>[2x]AGTYNYGEALQKSIMFYEFQRSGDLPADKRDNWRDDSGMKDGSDVGVDLTGGWYDAGDHVKFNLPMSYTSAMLAWSLYEDKDAYDKSGQTKYIMDGIKWANDYFIKCNPTPGVYYYQVGDGGKDHSWWGPAEVMQMERPSFKVDASKPGSAVCASTAASLASAAVVFKSSDPTYAEKCISHAKNLFDMADKAKSDAG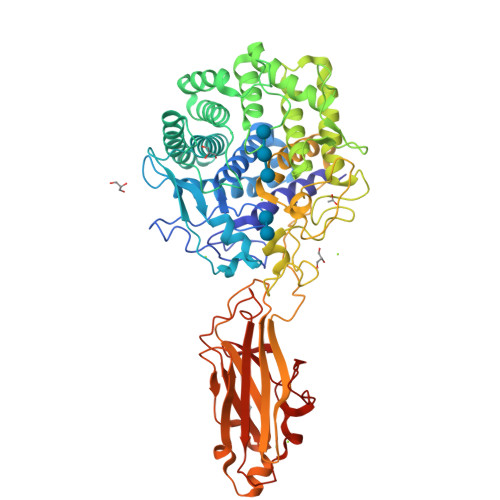YTAASGYYSSSSFYDDLSWAAVWLYLATNDSTYLDKAESYVPNWGKEQQTDIIAYKWGQCWDDVHYGAELLLAKLTNKQLYKDSIEMNLDFWTTGVNGTRVSYTPKGLAWLFQWGSLRHATTQAFLAGVYAEWEGCTPSKVSVYKDFLKSQIDYALGSTGRSFVVGYGVNPPQHPHHRTAHGSWTDQMTSPTYHRHTIYGALVGGPDNADGYTDEINNYVNNEIACDYNAGFTGALAKMYKHSGGDPIPNFKAIEKITNDEVIIKAGLNSTGPNYTEIKAVVYNQTGWPARVTDKISFKYFMDLSEIVAAGIDPLSLVTSSNYSEGKNTKVSGVLPWDVSNNVYYVNVDLTGENIYPGGQSACRREVQFRIAAPQGTTYWNPKNDFSYDGLPTTSTVNTVTNIPVYDNGVKVFGNEP> MKPYQRQFIEFALNKQVLKFGEFTLKSGRKSPYFFNAGLFNTGRDLALLGRFYAEALVDSGIEFDLLFGPAYKGIPIATTTAVALAEHHDKDLPYCFNRKEAKDHGEGGSLVGSALQGRVMLVDDVITAGTAIRESMEIIQAHGATLAGVLISLDRQERGRGEISAIQEVERDYGCKVISIITLKDLIAYLEEKPDMAEHLAAVR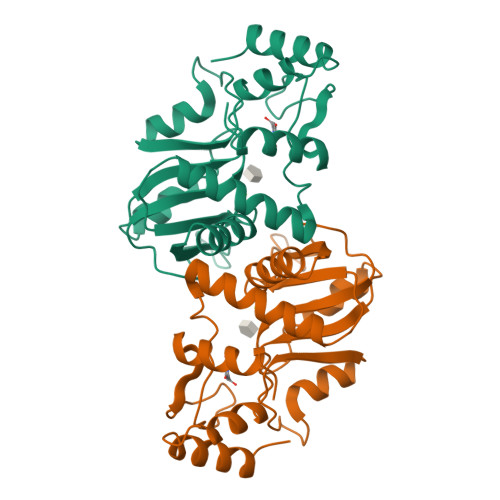AYREEFGV The transient receptor potential channel TRPM7 is a master regulator of the organismal balance of divalent cations that plays an essential role in embryonic development, immune responses, cell mobility, proliferation, and differentiation. TRPM7 represents a master regulator of the cellular balance of divalent cations and mediates uptake of Zn2+, Mg2+ and Ca2+, which is required for the normal prenatal development and healthy adulthood. The TRPM7 structure represents a tetramer assembled of four identical subunits, with the overall architecture reminiscent of other TRPM channels. Each TRPM7 subunit consists of an intracellular N-terminal domain (NTD, residues 1–789), transmembrane domain (TMD, 839–1146), and cytosolic C-terminal domain (CTD, 1157–1230).

The NTD includes four melastatin homology regions (MHR1-4).

> SQKSWIESTLTKRECVYIIPSSKDPHRCLPGCQICQQLVRCFCGRLVKQHACFTASLAMKYSDVKLGEHFNQAIEEWSVEKHTEQSPTDAYGVINFQGGSHSYRAKYVRLSYDTKPEIILQLLLKEWQMELPKLVISVHGGMQKFELHPRIKQLLGKGLIKAAVTTGAWILTGGVNTGVAKHVGDALKEHASRSSRKICTIGIAPWGVIENRNDLVGRDVVAPYQTLLNPLSKLNVLNNLHSHFILVDDGTVGKYGAEVRLRRELEKTINQQRIHARIGQGVPVVALIFEGGPNVILTVLEYLQESPPVPVVVCEGTGRAADLLAYIHKQTEEGGNLPDAAEPDIISTIKKTFNFGQSEAVHLFQTMMECMKKKELITVFHIGSEDHQDIDVAILTALLKGTNASAFDQLILTLAWDRVDIAKNHVFVYGQQWLVGSLEQAMLDALVMDRVSFVKLLIENGVSMHKFLTIPRLEELYNTKQGPTNPMLFHLIRDVKQGNLPPGYKITLIDIGLVIEYLMGGTYRCTYTRKRFRLIYNSLGGNNRRSGRNTSSSTPQLRKSHETFGNRADKKEKMRHNHFIKTAQPYRPKMDASMEEGKKKRTKDEIVDIDDPETKRFPYPLNELLIWACLMKRQVMARFLWQHGEESMAKALVACKIYRSMAYEAKQSDLVDDTSEELKQYSNDFGQLAVELLEQSFRQDETMAMKLLTYELKNWSNSTCLKLAVSSRLRPFVAHTCTQMLLSDMWMGRLNMRKNSWYKVILSILVPPAILMLEYKTKAEMSHIPQSQDAHQMTMEDSENNFHNITEEIPMEVFKEVKILDSSDGKNEMEIHIKSKKLPITRKFYAFYHAPIVKFWFNTLAYLGFLMLYTFVVLVKMEQLPSVQEWIVIAYIFTYAIEKVREVFMSEAGKISQKIKVWFSDYFNVSDTIAIISFFVGFGLRFGAKWNYINAYDNHVFVAGRLIYCLNIIFWYVRLLDFLAVNQQAGPYVMMIGKMVANMFYIVVIMALVLLSFGVPRKAILYPHEEPSWSLAKDIVFHPYWMIFGEVYAYEIDVCANDSTLPTICGPGTWLTPFLQAVYLFVQYIIMVNLLIAFFNNVYLQVKAISNIVWKYQRYHFIMAYHEKPVLPPPLIILSHIVSLFCCVCKRRKKDKTSDGPKLFLTEEDQKKLHDFEEQCVEMYFDEKDDKFNSGSEERIRVTFERVEQMSIQIKEVGDRVNYIKRSLQSLDSQIGHLQDLSALTVDTLKTLTAQKASEASKVHNEITRELSISKHLAQNLID> SEFELGAPATRSAGQQATVDRLRTQVTGFLSGALGKLQALSAQNMDPELAQFRVLDVDRAIMPLLIVAENARNPGLN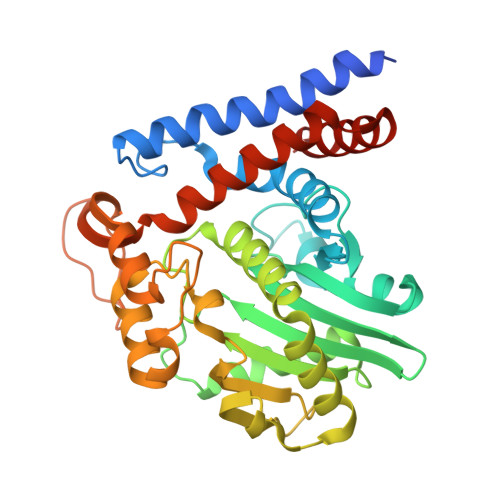LVPLHMDMAEDEEVRTQPPMAGSRHIAEFVASARPGRYRAVIDDGSHTRAADIRKDASGTSVIVVDPLRKEKDESAYVDYADNVNMEFGEHAKCAFIPVDIQKSFFDCRILSLSLALKMHDKDDAFAAFHETLRNGGDPSHHVSRAQQTEELGATLVLDGAPLVDARMMKHGQAASSVSRYLGNHPEQSTVPVNKRNETLGERTTRHLVKRKVRNRADSEGRVTSGETKEITFSNSVEQKRIALLNRAASYVNSAPPPVVMRMAKLLQDSLLDTN N-[(4-fluorophenyl)methyl]-2-{(1R)-5-[(methylcarbamoyl)amino]-2',4'-dioxo-2,3-dihydro-3'H-spiro[indene-1,5'-[1,3]oxazolidin]-3'-yl}-N-[(2S)-1,1,1-trifluoropropan-2-yl]acetamide | C25 H24 F4 N4 O5 | 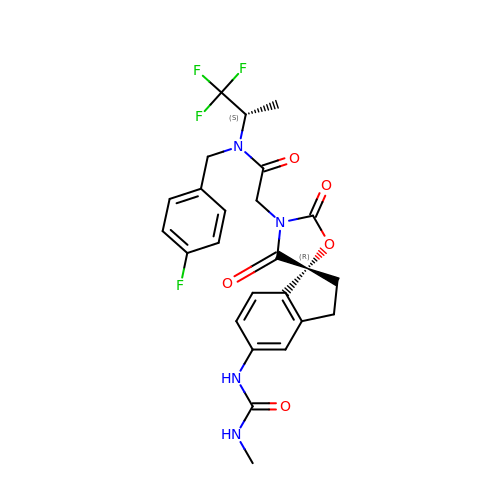VRVJKILQRBSEAG-LFPIHBKWSA-N> MASVHGTTYELLRRQGIDTVFGNPGSNELPFLKDFPEDFRYILALQEACVVGIADGYAQASRKPAFINLHSAAGTGNAMGALSNAWNSHSPLIVTAGQQTRAMIGVEALLTNVDAANLPRPLVKWSYEPASAAEVPHAMSRAIHMASMAPQGPVYLSVPYDDWDKDADPQSHHLFDRHVSSSVRLNDQDLDILVKALNSASNPAIVLGPDVDAANANADCVMLAERLKAPVWVAPSAPRCPFPTRHPCFRGLMPAGIAAISQLLEGHDVVLVIGAPVFRYHQYDPGQYLKPGTRLISVTCDPLEAARAPMGDAIVADIGAMASALANLVEESSRQLPTAAPEPAKVDQDAGRLHPETVFDTLNDMAPENAIYLNESTSTTAQMWQRLNMRNPGSYYFCAAGG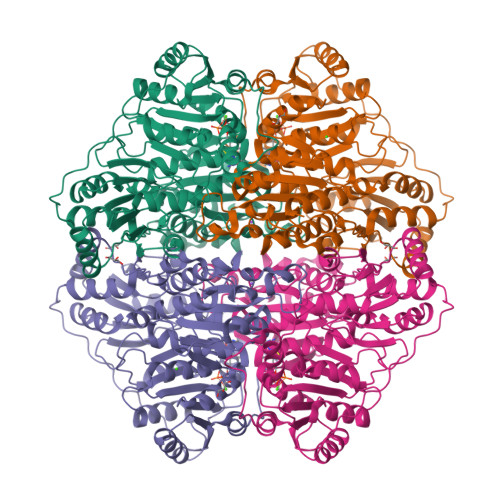NGFALPAAIGVQLAEPERQVIAVIGDGSANYSISALWTAAQYNIPTIFVIMNNGTYGALRWFAGVLEAENVPGLDVPGIDFRALAKGYGVQALKADNLEQLKGSLQEALSAKGPVLIEVSTVSPVKRSHHHHHH>[2x]DCNILQRLKVKMQWAKAYGFGTERAKFGNSLWTSIFNYAPDARDLFKSVKSEDMRSPQFKAHIARVIGGLDRVISMFDNEDALNADLEHLKSQHDPRGLDALNFVVFGKALFATVGGQF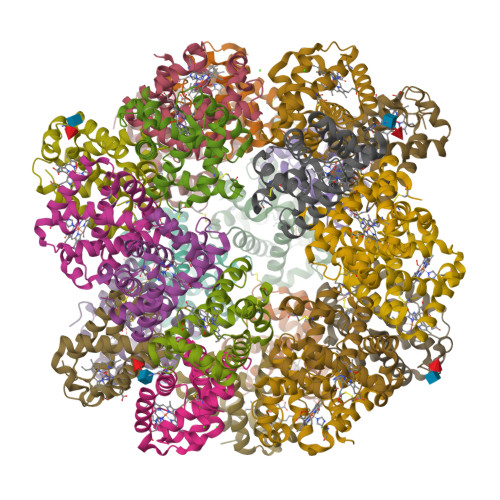GVCFDLPAWESCYKVIAMGITGNDMFS;>[2x]SECGPLQRLKVKRQWAEAYGSGNGREEFGHFIWANVFKVAPSARDMFKRVRGDNIYTPAFRAHATRVLGGLDMCVALLDDESVLNTQLAHLASQHSSRGVSAEQYNVVEHAVMMGVEHEIGQNVFDKDAWQACLDVITSGIQGN;>SSNSCTTEDRREMQLMWANVWSAQFTGRRLAIAQAVFKDLFAHVPDAVGLFDRVHGTEIDSSEFKAHCIRVVNGLDSAIGLLSDPSTLNEQLSHLATQHQERAGVTKGGFSAIAQSFLRVMPQVASCFNPDAWSRCFNRITNGMTEGLAE[2x];>[2x]SEFCSEADATIVIKQWNQIYNAGIGAKSRWTMGNEIFSSLFKLKPESEVLFNNVNVANMSSGAFHAHTVRVLSGLDMGINYLNDAGTLTSLTAHLAAQHVARTGLKAVYFDAMGKVLMTVLPSLIDNFNPDAWRNCLLPLKNAIAKGLP N4-HYDROXY-2-ISOBUTYL-N1-(9-OXO-1,8-DIAZA-TRICYCLO[10.6.1.013,18]NONADECA-12(19),13,15,17-TETRAEN-10-YL)-SUCCINAMIDE 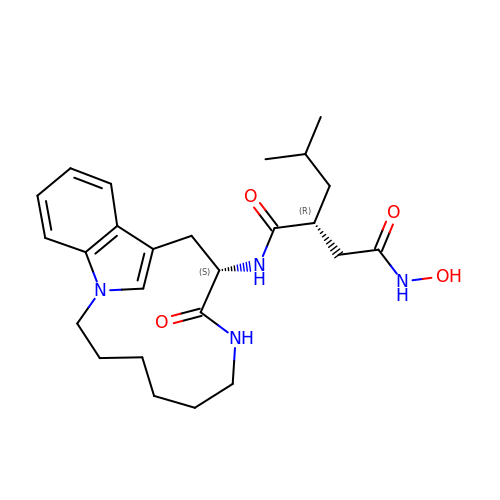| C25 H36 N4 O4 | GCBPAPVOMPJQHK-NQIIRXRSSA-N Triptorelin is a decapeptide with uncharged N- and C-termini pE1–H2–W3–S4–Y5–(D)W6–L7–R8–P9–G10–NH2 that contains three aromatic side chains (Y5, W3 and W6), and three ionizable residues, R8 and Y5 (pKa>10) and a histidine, H2 (pKa=6.1 in water). In this letter, we report on a decapeptide that self-assembles into either 50 nm diameter nanotubes at high pH or 10.7 nm diameter nanotubes at low pH. The peptide conformation switches from a globular one at pH>7.5 to an extended one at pH<6.5. All together, these results show that the peptide conformation, the peptide molecular packing and the assembly morphology of the triptorelin self-assemblies depend on the protonation state of the peptide single histidine, H2.

To obtain insights into the nanotube structure at atomic level, the peptide was crystallized as used for amyloid structure determination. Small triptorelin crystals were formed in the presence of phosphate anions that are larger than acetate. By optimizing the crystallization conditions large single crystals diffracting up to 0.85 Å resolution were obtained. The high-pH crystal structure obtained at 0.85 Å resolution reveals a histidine-serine H-bond and histidine-aromatic interactions, whereas the low-pH molecular structure demonstrates these key interactions have disappeared, likely in favour of cation-π proximities. Hence, the 25-Å-thick bilayer observed in the crystal structure (fully compatible with the 26 Å determined by SAXS) is essentially maintained by aromatic stacking, as shown by the side view of the bilayer and in agreement with the low β-sheet content observed by ATR-FTIR. The histidine tautomer in the crystal and in the nanotubes is the τ tautomer. Remarkably, the histidine residue is part of a hydrophobic aromatic cluster and its orientation is locked by two strong hydrogen bonds with the S4OH group and the backbone amine at distances (nitrogen to proton) of 2.1 and 2.21 Å, respectively. Finally, in agreement with both ATR-FTIR and Raman data, almost no direct intra- or inter-molecular hydrogen bonds stabilize the peptide conformation or the peptide packing except within the type II′ β-turn induced by the (D)W6. At high pH, the monocationic peptide with a single-positive charge on R8 is coiled at the level of the five contiguous residues H2–W3–S4–Y5–(D)W6 with five intramolecular interactions among them (right). At high pH, H2 is involved in an intramolecular interaction network, that is, two strong H-bond H2–S4 and π– π interactions between H2 and Y5 (intra- and inter-molecularly) and between H2 and W3.

>[4x]QHWSYWLRPGX> GLSAAQRQVVASTWKDIAGSDNGAGVGKECFTKFLSAHHDMAAVFGFSGASDPGVADLGAKVLAQIGVAVSHLGDEGKMVAEMKAV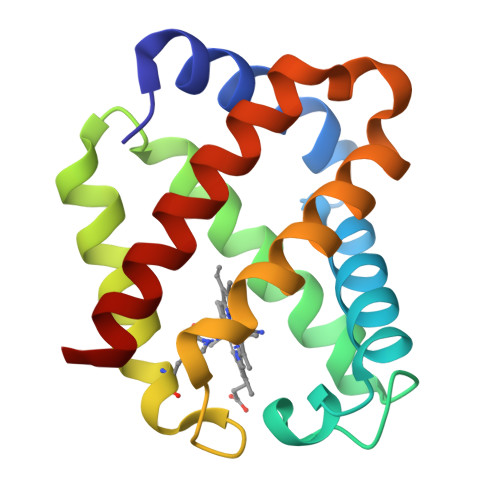GVRHKGYGNKHIKAEYFEPLGASLLSAMEHRIGGKMNAAAKDAWAAAYADISGALISGLQS7-[(3-CHLOROBENZYL)OXY]-2-OXO-2H-CHROMENE-4-CARBALDEHYDE | C17 H11 Cl 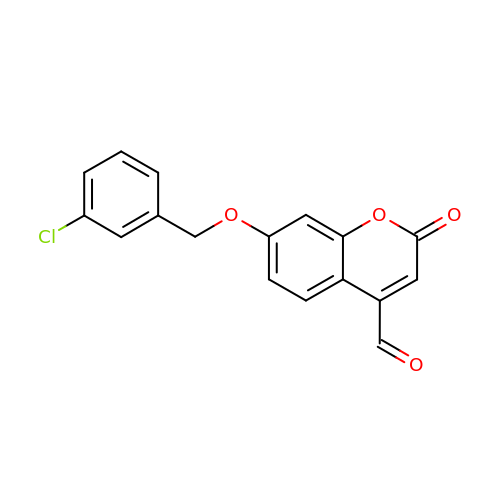O4 | ZOCADHRNWNJARU-UHFFFAOYSA-N> MKLSSACAIALLAAQAAGASIKHRINGFTLTEHSDPAKRELLQKYVTWDDKSLFINGERIMIFSGEFHPFRLPVKELQLDIFQKVKALGFNCVSFYVDWALVEGKPGEYRADGIFDLEPFFDAASEAGIYLLARPGPYINAESSGGGFPGWLQRVNGTLRSSDKAYLDATDNYVSHVAATIAKYQITNGGPIILYQPENEYTSGCCGVEFPDPVYMQYVEDQARNAGVVIPLINNDASASGNNAPGTGKGAVDIYGHDSYPLGFDCANPTVWPSGDLPTNFRTLHLEQSPTTPYAIVQFQGGSYDPWGGPGFAACSELLNNEFERVFYKNDFSFQIAIMNLYMIFGGTNWGNLGYPNGYTSYDYGSAVTESRNITREKYSELKLLGNFAKVSPGYLTASPGNLTTSGYADTTDLTVTPLLGNSTGSFFVVRHSDYSSEESTSYKLRLPTSAGSVTIPQLGGTLTLNGRDSKIHVTDYNVSGTNIIYSTAEVFTWKKFADGKVLVLYGGAGEHHELAISTKSNVTVIEGSESGISSKQTSSSVVVGWDVSTTRRIIQVGDLKILLLDRNSAYNYWVPQLATDGTSPGFSTPEKVASSIIVKAGYLVRTAYLKGSGLYLTADFNATTSVEVIGVPSTAKNLFINGDKTSHTVDKNGIWSATVDYNAPDISLPSLKDLDWKYVDTLPEIQSSYDDSLWPAADLKQTKNTLRSLTTPTSLYSSDYGFHTGYLLYRGHFTATGNESTFAIDTQGGSAFGSSVWLNGTYLGSWTGLYANSDYNATYNLPQLQAGKTYVITVVIDNMGLEENWTVGEDLMKTPRGIL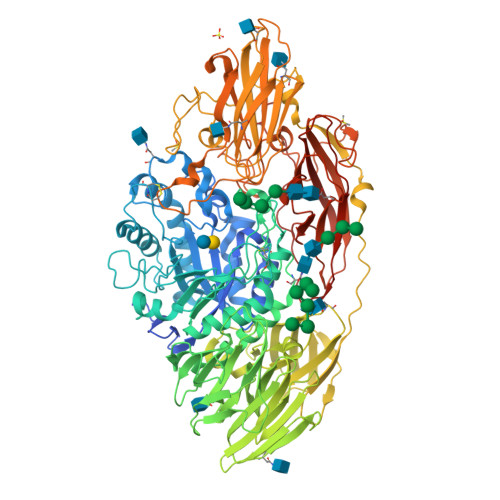NFLLAGRPSSAISWKLTGNLGGEDYEDKVRGPLNEGGLYAERQGFHQPEPPSQNWKSSSPLEGLSEAGIGFYSASFDLDLPKGWDVPLFLNIGNSTTPSPYRVQVYVNGYQYAKYISNIGPQTSFPVPEGILNYRGTNWLAVTLWALDSAGGKLESLELSYTTPVLTALGEVESVDQPKYKKRKGAYHHHHHH N-[(2R)-2-{[(2S)-2-(1,3-benzoxazol-2-yl)pyrrolidin-1-yl]carbonyl}hexyl]-N-hydroxyformamide 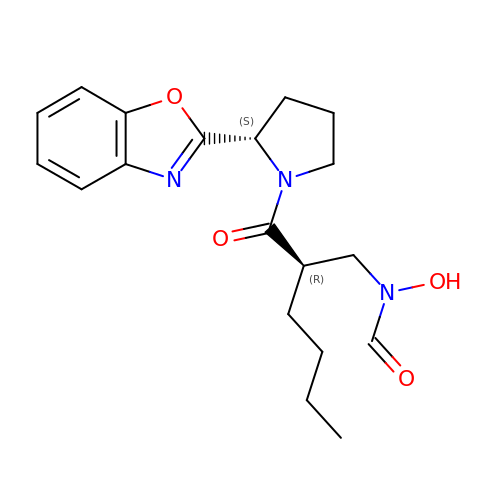| C19 H25 N3 O4 | QDDZLTVSNABZIK-ZBFHGGJFSA-N(2S,3R,4R,5R,6R)-2-[(2S,3R,4S,5R,6S)-6-(hydroxymethyl)-2-[[(2R,4R)-2-(4-hydroxyphenyl)-4,5-bis(oxidanyl)-3,4-dihydro-2H-chromen-7-yl]oxy]-4,5-bis(oxidanyl)oxan-3-yl]oxy-6-methyl-oxane-3,4,5-triol 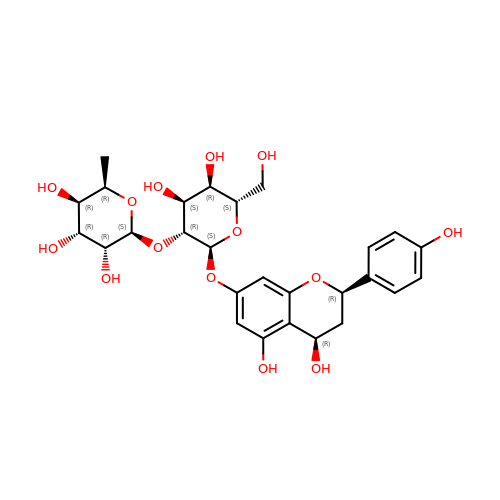| C27 H34 O14 | AFQQXXZQSJSQTD-REMLSPIZSA-N The Drosophila tumour necrosis factor (TNF) ligand-receptor system consists of a unique ligand, Eiger (Egr), and two receptors, Grindelwald (Grnd) and Wengen (Wgn), and therefore provides a simple system for exploring the interplay between ligand and receptors, and the requirement for Grnd and Wgn in TNF/Egr-mediated processes. Here, we report the crystallographic structure of the extracellular domain (ECD) of Grnd in complex with Egr, a high-affinity hetero-hexameric assembly reminiscent of human TNF:TNFR complexes. Here we show that trimeric Egr ligands assemble in hetero-hexamers with both Grnd and Wgn, with Grnd displaying nanomolar binding affinity for Egr, which is 3-orders of magnitude higher than that for Wgn. Altogether, our data provide insight into ligand-mediated activation of Grnd and suggest that distinct affinities of TNF ligands for their receptors promote different and non-redundant cellular functions.

To uncover the organizational principles of the Grnd:Egr interaction, we first determined the crystallographic structure of the extracellular portion of Grnd. Therefore, we further trimmed its boundaries by limited proteolysis with trypsin to a shorter fragment, which was assigned by mass spectrometry to Grnd30–81. The proteolytically defined Grnd30–81 readily yielded crystals diffracting to 0.92 Å resolution. The structure was solved by S-SAD, and refined to a Rfree of 0.16 and good stereochemistry. The final model includes residues 34–81 of Grnd, which we will refer to as Grnd-ECD hereon. The structure of Grnd-ECD consists of an N-terminal β-hairpin followed by two C-terminal antiparallel α-helices, with the 8 cysteines engaged in four disulfide bonds, with a topology that is reminiscent of the CRD fold seen in structurally known TNFRs. The C-terminus of the Grnd-CRD folds in a C2 helix-loop-helix module, organized in a nested pattern of disulfide bridges, according to the consensus sequence Cys57-x3-Cys61-x6-x5-Cys73-x3-Cys77 (where x is any given amino acids, and the subscript n indicates the number of residues). Although X2 and C2 modules are common features of TNFRs, Grnd-ECD is the first example of a TNFR fold combining the two together, with the side-chain of Phe46 fitting in between the two. A major finding of our structural characterization is that, in spite of the poor sequence homology, the ECD of Grnd adopts a cysteine-rich domain fold consisting of a X2 β-hairpin followed by a helical C2 module, in a combination that has not been observed in TNFR domains so far. The reciprocal orientation of the Grnd X2-C2 modules resembles that observed in single CRDs of human TNFRs such as TACI, BCMA and Fn14 and the fourth CRD of TNFR1, with the conserved Phe46Grnd side-chain packing between the two.

> GESRDCHGTICHPVNEFCYVATERCHPCIEVCNNQTHNYDAFLCAKECSAYK>MEAPAAVVTGAAKRIGRAIAVKLHQTGYRVVIHYHNS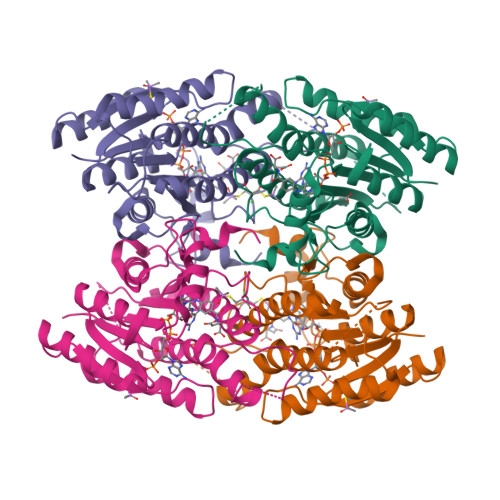AEAAVSLADELNKERSNTAVVCQADLTNSNVLPASCEEIINSCFRAFGRCDVLVNNASAFYPTPLVQGDHEDNSNGKTVETQVAELIGTNAIAPFLLTMSFAQRQKGTNPNCTSSNLSIVNLCDAMVDQPCMAFSLYNMGKHALVGLTQSAALELAPYGIRVNGVAPGVSLLPVAMGEEEKDKWRRKVPLGRREASAEQIADAVIFLVSGSAQYITGSIIKVDGGLSLVHA[4x]>MNTPEHMTAVVQRYVAALNAGDLDGIVAL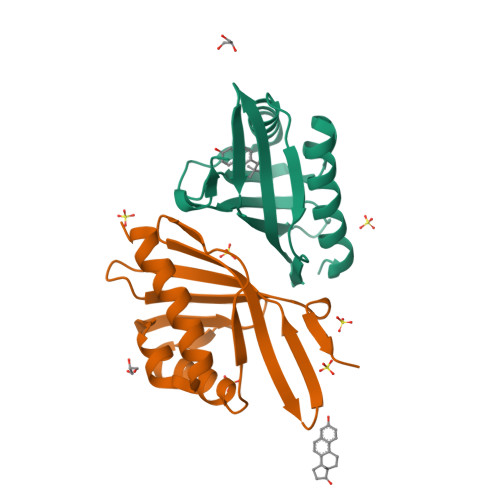FADDATVEHPVGSEPRSGTAAIREFYANSLKLPLAVELTQEVRAVANEAAFAFTVSFEYQGRKTVVAPINHFRFNGAGKVVSMRALFGEKNIHAGA[4x]> AMVSSSCSSIPKMPVTPLSLVTRHVAIIGAGAAGLVTARELRREGHTTTIFERGSSIGGTWIYTPDTEPDPMSQDSSRPIVHSSLYKSLRTNLPREVMGFLDYPFVEKTNGGDRRRFPGHEEVLDYLERFGREFGVSREVGMEKEVVRVDMEQGGKWTVKWKGKDGGGGEEGFDAVVVCNGH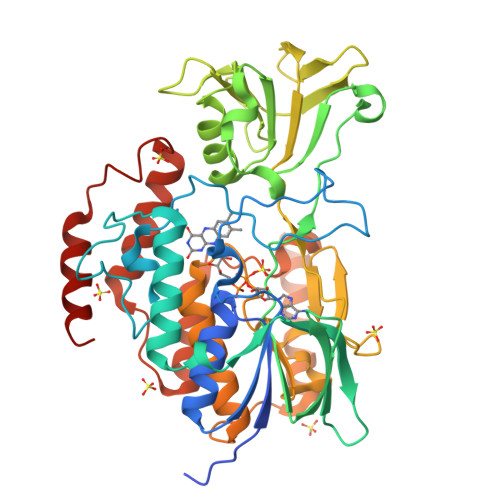YTEPRFAEIPGIDVWPGKQMHSHNYRIPEPFHDQVVVIIGSSASAVDISRDVARFAKEVHIANRSITEGTPAKQPGYDNMWLHSMIKITHNDGSVVFHDGCSVHVDVIMHCTGYVYNFPFLNTNGIVTVDDNRVGPLYKHVFPPLLAPSLSFVGIPWKIVPFPLCELQSKWIAAVLSGRISLPTKKEMMEDVEAYYKQMEAAGIPKRYTHNIGHNQFDYDDWLANECGYSCIEEWRRLMYKEVSKNRKERPESYRDEWDDDHLVAQARETFSKFLS4-[5-[(2~{S},3~{R},4~{R},5~{S},6~{R})-6-(hydroxymethyl)-3,4,5-tris(oxidanyl)oxan-2-yl]-4~{H}-1,2,4-triazol-3-yl]benzoic 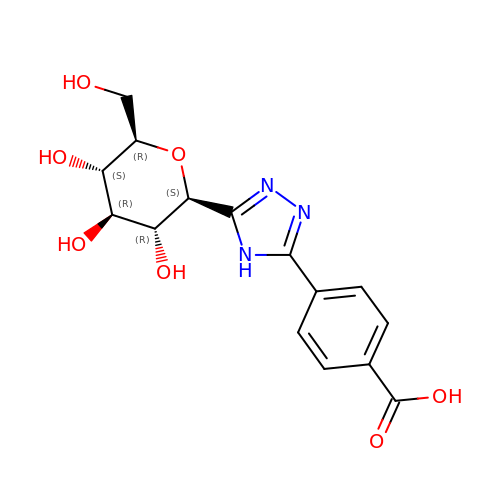acid | C15 H17 N3 O7 | UYSDRGPJXJKBOO-RMPHRYRLSA-N> LYFSRDAYWEKLYVDQAAGTPLLYVHALRDAPEEVPSFRLGQHLYGTYRTRLHENNWIRIQEDTGLLYLQRSLDHSSWEKLSVRNRGFPLLTVYLKVFLSPTSLREGECQWPGCARVYFSFFNTSFPACSSLKPRELCFPETRPSFRIRENRP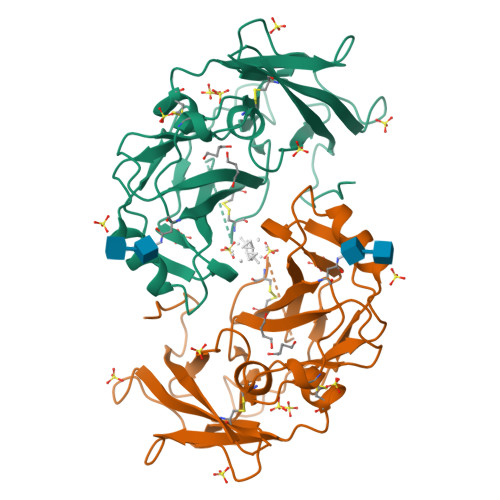PGTFHQFRLLPVQFLCPQISVAYRLLEGEGLPFRSAPDSLEVSTRWALDREQREKYELVAVCTVHAGAREEVVMVPFPVTVYDEDDSAPEFEN>[6x]XQIAAIKEAIAAIKQQIAAIKXA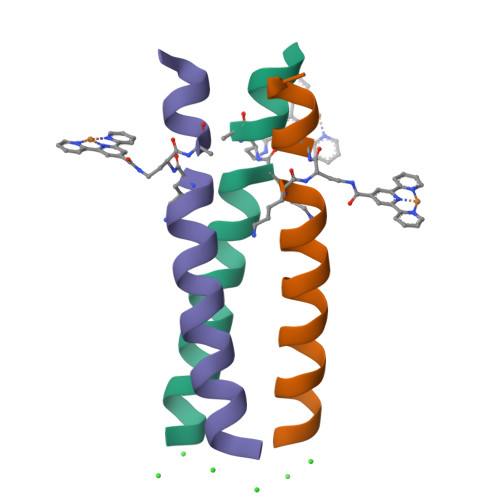IAAIKQX>[2x]GSVDDHHHGPKQVMVLKVTEPFTYDLKEDKRMFHATVATETEFFRVKVFDTALKSKFIPRNIIAISDYFGCNGFLEIYRASCVSD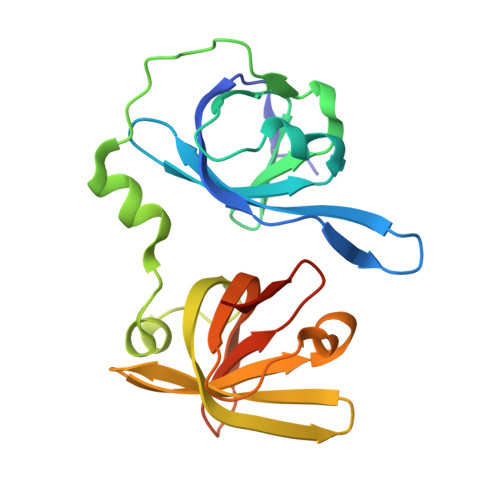VNVNPTMVISNTLRQRANATPKISYLFSQARGTFVSGEYLVNKKTERNKFIYYGIGDDTGKMEVVVYGRLTNVRCEPGSKLRLVCFELTSTEDGWQLRSVRHSYMQVINARKAAAS>AEEFPVPNGFESAYREVDGVKLHYVKGGQGPLVMLVHGFGQTWYEWHQLMPELAKRFTVIAPDLPGLGQSEPPKTGYSGEQVAVYLHKLARQFSPDRPFDLVAHDIGIWNTYPMVVKNQADIARLVYMQAPIPDARIYRFPAFTAQGESLVWHFSFFAADDRLAETLIAGKERFFLEHFIKSHASNTEVFSERLLDLYARSYAKPHSLNASFEYYRALNESVRQNAELAKTRLQMPTMTLAGGGHGGMGTFQLEQMKAYAEDVE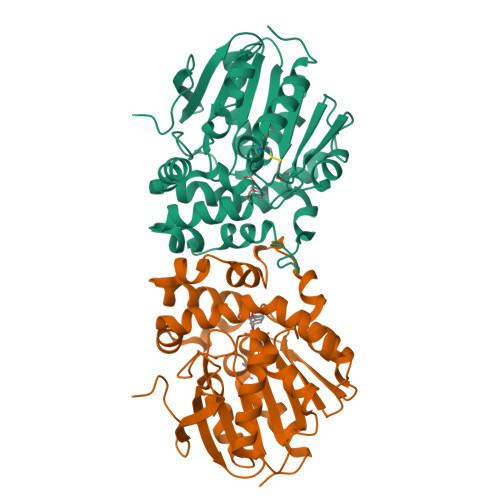GHVLPGCGHWLPEECAAPMNRLVIDFLSRGRHHHHHH[4x]> MAEAGLRGWLLWALLLRLAQSEPYTTIHQPGYCAFYDECGKNPELSGSLMTLSNVSCLSNTPARKITGDHLILLQKICPRLYTGPNTQACCSAKQLVSLEASLSITKALLTRCPACSDNFVNLHCHNTCSPNQSLFINVTRVAQLGAGQLPAVVAYEAFYQHSFAEQSYDSCSRVRVPAAATLAVGTMCGVYGSALCNAQRWLNFQGDTGNGLAPLDITFHLLEPGQAVGSGIQPLNEGVARCNESQGDDVATCSCQDCAASCPAIARPQALDSTFYLGQMPGSLVLIIILCSVFAVVTILLVGFRVAPARDKSKMVDPKKGTSLSDKLSFSTHTLLGQFFQGWGTRVASWPLTILVLSVIPVVALAAGLVFTELTTDPVELWSAPNSQARSEKAFHDQHFGPFFRTNQVILTAPNRSSYRYDSLLLGPKNFSGILDLDLLLELLELQERLRHLQVWSPEAQRNISLQDICYAPLNPDNTSLYDCCINSLLQYFQNNRTLLLLTANQTLMGQTSQVDWKDHFLYCANAPLTFKDGTALALSCMADYGAPVFPFLAIGGYKGKDYSEAEALIMTFSLNNYPAGDPRLAQAKLWEEAFLEEMRAFQRRMAGMFQVTFMAERSLEDEINRTTAEDLPIFATSYIVIFLYISLALGSYSSWSRVMVDSKATLGLGGVAVVLGAVMAAMGFFSYLGIRSSLVILQVVPFLVLSVGADNIFIFVLEYQ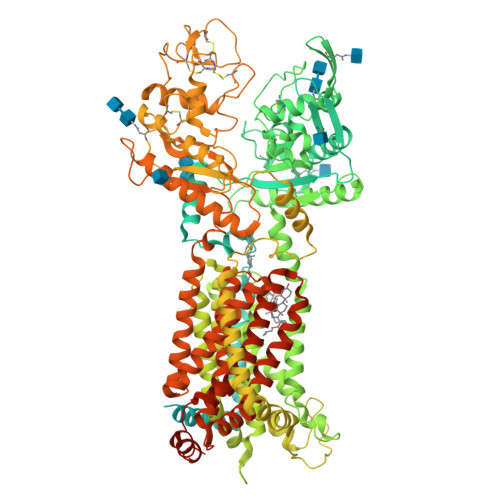RLPRRPGEPREVHIGRALGRVAPSMLLCSLSEAICFFLGALTPMPAVRTFALTSGLAVILDFLLQMSAFVALLSLDSKRQEASRLDVCCCVKPQELPPPGQGEGLLLGFFQKAYAPFLLHWITRGVVLLLFLALFGVSLYSMCHISVGLDQELALPKDSYLLDYFLFLNRYFEVGAPVYFVTTLGYNFSSEAGMNAICSSAGCNNFSFTQKIQYATEFPEQSYLAIPASSWVDDFIDWLTPSSCCRLYISGPNKDKFCPSTVNSLNCLKNCMSITMGSVRPSVEQFHKYLPWFLNDRPNIKCPKGGLAAYSTSVNLTSDGQVLTSRFMAYHKPLKNSQDYTEALRAARELAANITADLRKVPGTDPAFEVFPYTITNVFYEQYLTILPEGLFMLSLCLVPTFAVSCLLLGLDLRSGLLNLLSIVMILVDTVGFMALWGISYNAVSLINLVSAVGMSVEFVSHITRSFAISTKPTWLERAKEATISMGSAVFAGVAMTNLPGILVLGLAKAQLIQIFFFRLNLLITLLGLLHGLVFLPVILSYVGPDVNPALALEQKRAEEAVAAVMVASCPNHPSRVSTADNIYVNHSFEGSIKGAGAISNFLPNNGRQF> MAQLTHINAAGEAHMVDVSAKAETVREARAEAFVTMRSETLAMIIDGRHHAGDVFATARIAGIQAAKRTWDLIPLCHPLMLSKVEVNLQAEPEHNRVRIE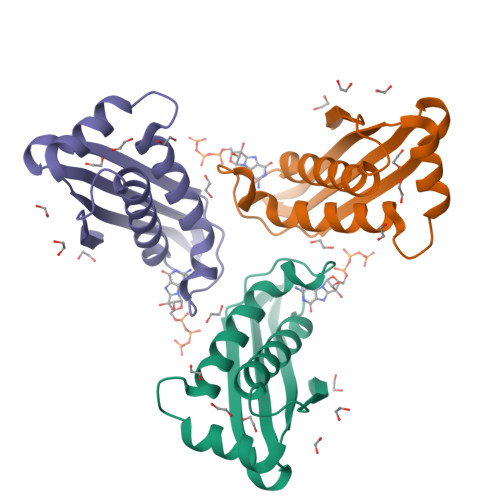TLCRLTGKTGVEMEALTAASVAALTIYDMCKAVQKDMVIGPVRLLAKSGGKSGDFKVEADD> VGWEQLLTTIARTI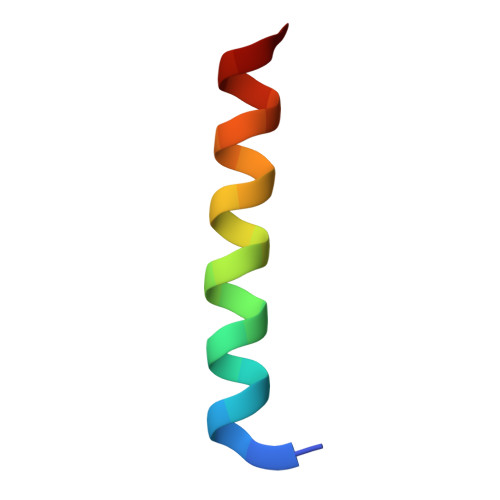NEVENQILTR Here we provide the structural and enzymatic characterization of the recently identified enzyme isolated from Pseudomonas pseudoalcaligenes dubbed OPHC2. OPHC2 belongs to the metallo-β-lactamase superfamily and exhibits an unusual thermal resistance and some OP degrading abilities. OPHC2 belongs to the metallo-β-lactamase superfamily and shares significant homology with other representatives such as MPH (identity = 48%; similarity = 58.6%), and lower sequence identity with the lactonases AiiA (17–18%) and AiiB (14%). We here show that OPHC2 hydrolyzes a broad range of esters, from phosphotriesters to the lactone dihydrocoumarin.

OPHC2 enzyme, as observed for MPH, crystallizes as a homodimer, and biochemical evidences suggests that this dimer exists in solution. This homodimer exhibits (i) a very important surface interaction, (ii) a high number of intermolecular hydrogen bonds and salt bridges. The monomer of OPHC2 is roughly globular with overall dimensions of approximately 44 Å×50 Å×37 Å. As for MPH, its structure could be described as an αβ/βα sandwich topology, typical of the metallo-β-lactamase superfamily. The superposition of OPHC2 with MPH and AiiA yields RMSD values for α-carbon atoms of 0.74 Å (over 213 residues) and 2.41 Å (over 105 residues), respectively. The active site of OPHC2 consists of a cavity with two metal cations: one buried (α metal) and one more solvent exposed (β metal). The catalytic center is composed of two metals bridging an activated water molecule as observed in MPH and AiiA structures, but also other esterases such as SsoPox or SisLac. OPHC2’s active site comprises a highly hydrophobic substrate binding pocket which thus seems well adapted for the accommodation of the hydrophobic molecules that comprise OPs. Comparison of both active site highlights amino acids differences in the leaving group pocket (e.g. Met188OPHC2 instead of Phe196MPH), in the side pockets (e.g Phe265OPHC2 instead of Leu273OPHC2 and Leu61OPHC2 instead of Arg72MPH, and the presence of an additional Phe263OPHC2 in the binding pocket), as well as the floppy region 168–210. The higher thermal stability of OPHC2, as compared to its closest known homologue MPH, may stem from a high dimer interface area and an intramolecular disulfide bridge.

>[5x]MRLFSLSTALSSAMIALVSLPLQAAAPAQQKTQVPGYYRMALGDFEVTALYDGYVDLPASLLKGIDDKDLQSLLARMFVASEKGVQTAVNAYLINTGDNLVLIDTGAAQCFGPTLGVVQTNLKASGYQPEQVDTVLLTHLHPDHACGLVNADGSPAYPNATVEVPQAEAEFWLDEATMAKAPEGMQGMFKMAQQAVAPYAKMNKLKPYKTEGELLPGVSLVASPGHTPGHTSYLFKSGGQSLLVWGDILLNHAVQFAKPEVVFEFDVDSDQARQSRQRILAEAATDKLWVAGAHLPFPGLGHVRKEAQGYAWVPVEFSPIRSDR> MFNQPPRFQNYFFQSYLLIYENTPVGSSITQLTAVDPDGEPLIFGVVGEEASRFFAVQENTGVVWLRQPLDRETKSEMQVVFSVSDSQGVVKDTVNIQIGDVNDNAPTFHNQPYTVNIPEDTSVGTSIFMVNATDPDQGTGGSVLFSFQPPSPFFSIDGARGIITVSRLLDYEVTSAYQLTVNATDQDKLHPLSSLANLAITLSDIQDRDLEHHHHHH;> MSSKSQDSDDWQYEECKLSRTGPPATIVAIDEESPNGTVLVENMQINGRAEDPHRTIS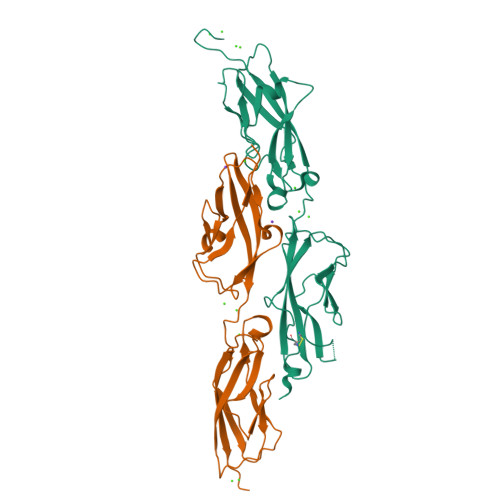LSLRDNYGHWVILDPVKQRLYLNSTGRVLDRDPPSYIHSIVVQVQCTNELVGTVILHEVRIVVRDRNDNPPRFQQPRYYVAINELTPVGTTIFSGFSGNNGAVDIDDGPNGQIEYTIQYNPYDPTANRTFDIPLTLSGSVVLRERLNYEEITRYLVIIQANDRAPDPKERLTATTTLTVDVLDGDDLGPLEHHHHHH4-(METHYLSULFANYL)-2-OXOBUTANOIC ACID | C5 H8 O3 S | 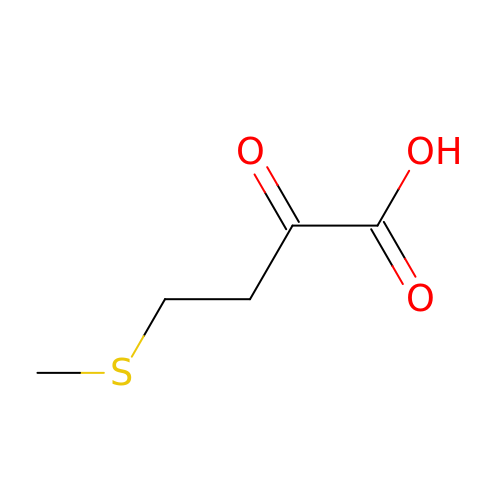SXFSQZDSUWACKX-UHFFFAOYSA-N>[2x]EPFSLPNLQTDEMSSSRWPNPLATLFADPNVAVAPQWQNGRCTLEGELLGTTPRNASWLNRFRGVSTAAVANQVLHLTLYEPDGSVFNPLSGAPAPEGFPDFTAQEYHLRAAGKVANTTGGGEIKSTDYTPALGGVKITAWDATGPSAGVEMTGQIESIGMENNTDFDVLPDYNGSAFDGSLNLAPPIVPLLPGETLLRFGTVPITTRRQSDPIRIISCALPQEWITWFLTHNFTALGDAALLRYRNQATGQLLFECKLYRSGFVVVNGVNVRTEFPMSGVFEFVSWVPNFFQLAPV

Noroviruses are highly contagious, infecting both humans and animals. The human norovirus capsid protruding (P) domain binds histo-blood group antigen (HBGA) co-factors for infection, and a recently discovered bat norovirus (GX) was also found to interact with HBGAs. In this study, we determined the P domain structures of four human noroviruses and one bat norovirus using X-ray crystallography to examine structural features linked to potential interspecies transmission. The principal structural difference was a variable length P2 subdomain loop (Loop A), which was located near the HBGA pocket.

The P domains of GII.9 (AY038599), GII.23 (KT290889), GII.27 (MG495077), GVIII (AJ844470), and GX (MF373609) were expressed in E.coli. The five P domains were structurally equivalent with a root mean square deviation for C-alpha atoms ranging between 0.586 Å (GII.23-GII.27) and 1.645 Å (GII.9-GX). Also, these residue side chains were properly positioned to bind the fucose moiety of HBGAs (structure not shown). These two equivalent residues were lacking in the GVIII and GX P domains; however, an aspartic acid (D367) was located nearby in the GX P domain. The cross-reactivity of the P domains was determined using direct ELISA with a broad-spectrum human norovirus Nanobody (Fc-NB26) that binds to a highly conserved region on the P domain. Fc-NB26 bound to the GVIII P domain at weaker concentrations than these GII genotypes, while Fc-NB26 did not bind to the GX P domain at any concentration tested. The GVIII P domain also had many Fc-NB26-binding residues, while most Fc-NB26-binding residues were absent in GX. Subsequently, the bat norovirus could be considered antigenically distinct from human GII noroviruses. In addition, the bat norovirus HBGA-binding site may be shifted from the regular GII HBGA pocket, as observed in other genogroups.>[4x]MKKLTSGPALPGKLADCTAQDLNRTELFLVEGDSAGGSAKQARDREYQAIMPLKGKILNTWEVSSDEVLASQEVHDISVAIGIDPDSDDLSQLRYGKICILADADSDGLHIATLLCALFVRHFRTLVKEGHVYVALPPLYRIDLGKEVYYAL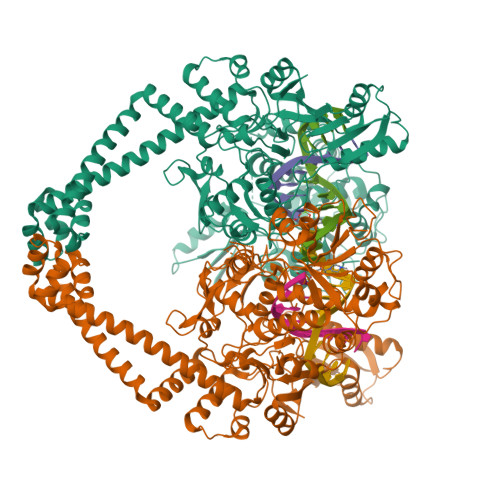TEEEKTGVLEQLKRKKGKPNVQRFKGLGEMNPMQLRETTLDPNTRRLVQLVISDEDEQQTTAIMDMLLAKKRSEDRRNWLQEKGDMADLEVEFMSDMAERLALHEFTENAYLNYSMYVIMDRALPFIGDGLKPVQRRIVYAMSELGLNASAKFKKSARTVGDVLGKYHPHGDSACYEAMVLMAQPFSYRYPLGDGQGNWGAPDDPKSFAAMRYTESRLSKYAELLLSELGQGTVDWVPNFDGTLQEPKMLPARLPNILLNGTTGIAVGMATDIPPHNLREVAKAAITLIEQPKTTLDELLDIVQGPDFPTEAEIITSRAEIRKIYQNGRGSVRMRAVWSKEDGAVVITALPHQVSGAKVLEQIAAQMRNKKLPMVDDLRDESDHENPTRLVIVPRSNRVDMEQVMNHLFATTDLEKSYRINLNMIGLDGRPAVKNLLEILSEWLVFRRDTVRRRLNHRLEKVLKRLHILEGLLVAFLNIDEVIEIIRTEDEPKPALMSRFGISETQAEAILELKLRHLAKLEEMKIRGEQSELEKERDQLQAILASERKMNNLLKKELQADADAFGDDRRSPLHEREEAKAMSHHHHHH>QSPAEIASFSPRPSLADSKAVLNQAVADLSVAHSILHQVHWYMRGRGFMIWHPKMDEYMEEIDGYLDEMSERLITLGGAPFSTLKEFSENSQLKEVLGDYNVTIEEQLARVVEVFRYLAALFQKGFDVSDEEGDSVTNDIFNVAKASIEKHIWMLQA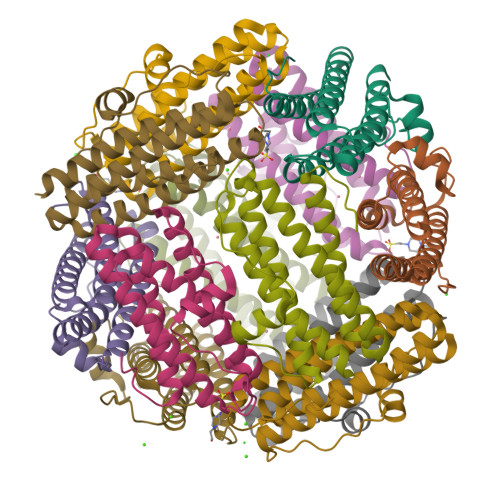ELGQAPKL[12x]> GSMDSDEGYNYEFDEDEECSEEDSGAEEEEDEDDDEPDDDTLDLGEVELVEPGLGVGGERDGLLCGETGGGGGSALGPGGGGGGGGGGGGGGPGHEQEEDYRYEVLTAEQILQHMVECIREVNEVIQNPATITRILLSHFNWDKEKLMERYFDGN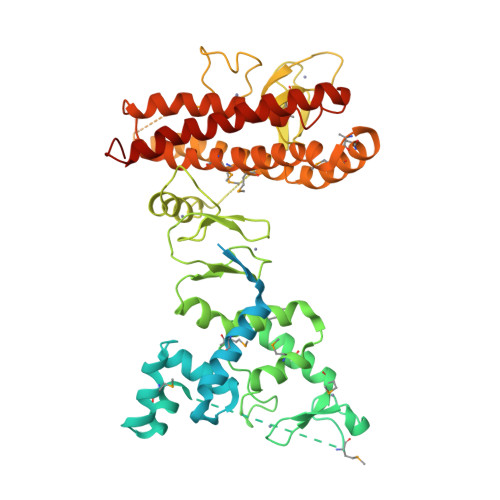LEKLFAECHVINPSKKSRTRQMNTRSSAQDMPCQICYLNYPNSYFTGLECGHKFCMQCWSEYLTTKIMEEGMGQTISCPAHGCDILVDDNTVMRLITDSKVKLKYQHLITNSFVECNRLLKWCPAPDCHHVVKVQYPDAKPVRCKCGRQFCFNCGENWHDPVKCKWLKKWIKKCDDDSETSNWIAANTKECPKCHVTIEKDGGCNHMVCRNQNCKAEFCWVCLGPWEPHGSAWYNCNRYNEDDAKAARDAQERSRAALQRYLFYCNRYMNHMQSLRFEHKLYAQVKQKMEEMQQHNMSWIEVQFLKKAVDVLCQCRATLMYTYVFAFYLKKNNQSIIFENNQADLENATEVLSGYLERDISQDSLQDIKQKVQDKYRYCESRRRVLLQHVHEGYEKDLWEYIED> AQSVPYGVSQIKAPALHSQGYTGSNVKVAVIDSGIDSSHPDLKVAGGASMVPSETNPFQDNNSHGTHVAGTVAALNNSIGVLGVAPSASLYAVKVLGADGSGQYSWIINGIEWAIANNMDVINMSLGGPSGSAALKAAVDKAVASGVVVVAAAGNEGTSGSSSTVGYPGKYPSVIAVGAVDSSNQRASFSSVGPELDVMAPGVSIQSTLPGNKYGAYNGTSMASPHVAGAAALILSKHPNWTNTQVRSSLENTTTKLGD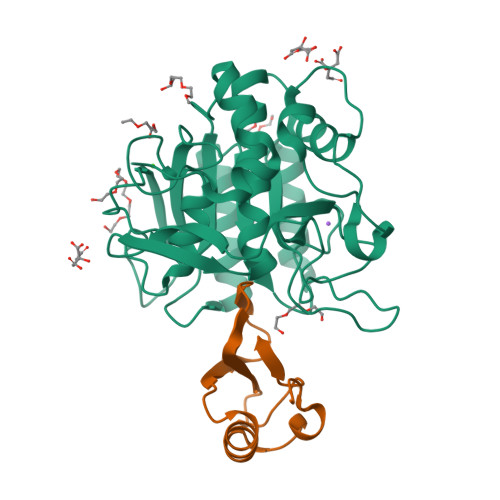SFYYGKGLINVQAAAQHHHHHH;> MKTEWPELVGKSVEEAKKVILQDKPAAQIIVLPVGTIVTFEYRIDRVRLFVDRLDNIAQVPRVG>[6x]MSLSYTTQQIIEKLRELKIVPVIALDNADDILPLADTLAKNGLSVAEITFRSEAAADAIRLLRANRPDFLIAAGTVLTAEQVVLAKSSGADFVVTPGLNPKIVKLCQDLNFPITPGVNNPMA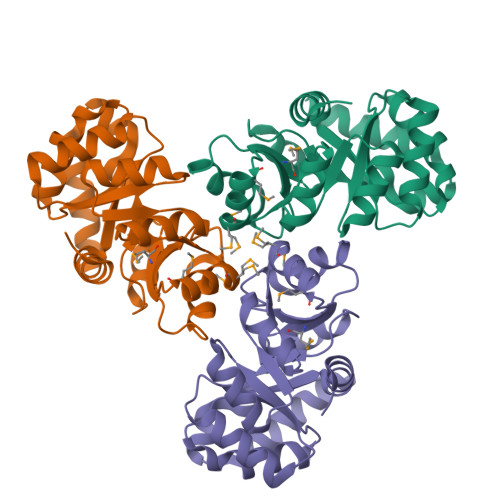IEIALEMGISAVKFFPAEASGGVKMIKALLGPYAQLQIMPTGGIGLHNIRDYLAIPNIVACGGSWFVEKKLIQSNNWDEIGRLVREVIDIIKEGGSHHHHHH>MANVDEAILKRVKGWAPYVDAKLGFRNHWYPVMFSKEINEGEPKTLKLLGENLLVNRIDGKLYCLKDRCLHRGVQLSVKVECKTKSTITCWYHAWTYRWEDGVLCDILTNPTSAQIGRQKLKTYPVQEAKGCVFIYLGDGDPPPLARDTPPNFLDDDMEILGKNQIIKSNWRLAVENGFDPSHIYIHKDSILVKDNDLALPLGFAPGGDRKQQTRVVDDDVVGRKGVYDLIGEHGVPVFEGTIGGEVVREGAYGEKIVANDISIWLPGVLKVNPFPNPDMMQFEWYVPIDENTHYYFQTLGKPCANDEERKKYEQEFESKWKPMALEGFNNDDIWAREAMVDFYADDKGWVNEILFESDEAIVAWRKLASEHNQGIQTQAHVSGLEHHHHHH[3x];>MNQIWLKVCAASDMQPGTIRRVNRVGAAPLAVYRVGDQFYATEDTCTHGIASLSEGTLDGDVIECPFHGGAFNVCTGMPASSPCTVPLGVFEVEVKEGEVYVAGEKKLEHHHHHH[3x]

Carbazole 1,9a-dioxygenase (CARDO), a RO member consists of catalytic terminal oxygenase (CARDO-O), ferredoxin (CARDO-F), and ferredoxin reductase. The mononuclear iron site activates dioxygen for reaction with the substrate, and the Rieske cluster transfers electrons to the mononuclear iron site during the catalytic cycle. In the present study, we determined the crystal structures of the reduced CAR-bound Oxy:Fd complex (Oxy: Fdred-CAR), oxygen-bound Oxy:Fd complex (Oxy: FdO2), and both CAR- and oxygen-bound Oxy:Fd complex (Oxy: FdCAR-O2) at 1.95, 1.85, and 2.0 Å resolution, respectively. All Oxy:Fd structures solved consist of one molecule of Oxy (comprising three subunits: chains A, B, and C) and three molecules of Fd (chains D, E, and F), and the asymmetric unit of the crystal contains one Oxy:Fd structure.

The structure obtained from air-treated Oxy: Fdred-CAR crystals during CAR-soaking seemed to bind with both CAR and dioxygen. The Fo-Fc map obtained during the course of crystallographic refinement of this structure showed a large residual density beside the nonheme iron, suggesting the existence of a dioxygen species. We refined the dioxygen species as described in the subsection “The Oxygen-Bound Complex Structure”, and the O–O distance was refined to approximately 1.5 Å. Therefore, the dioxygen species was likely a peroxide species. In chains B and C, the locations of dioxygen species were similar to those of the dioxygen-bound NDO-O with indole (side-on fashion), which indicates that the average bond lengths between mononuclear iron–Asp333OD1 and –Asp333OD2 were both approximately 1.8 Å and bound in a side-on fashion. The electron density of the dioxygen molecule at the active site of chain A was identical to that of Oxy: FdO2 (the bond lengths between mononuclear iron and oxygen atoms of Asp333 were 2.6 Å and 2.0 Å, respectively, in an end-on fashion). In addition, the electron density of CAR was not found in the active site of chain A. The average distances between peroxide O1 atom–CAR C9a atom and peroxide O2 atom–CAR C1 atom were both approximately 2.9 Å. This binding manner agrees with the fact that CARDO-O catalyzes the angular dioxygenation for CAR. Structural comparison of Oxy: FdO2 and Oxy: FdCAR-O2 demonstrated the possibility that regulation by the substrate ensures that reactive oxygen species bind to the desirable position in an appropriate side-on fashion.>[12x]GGGS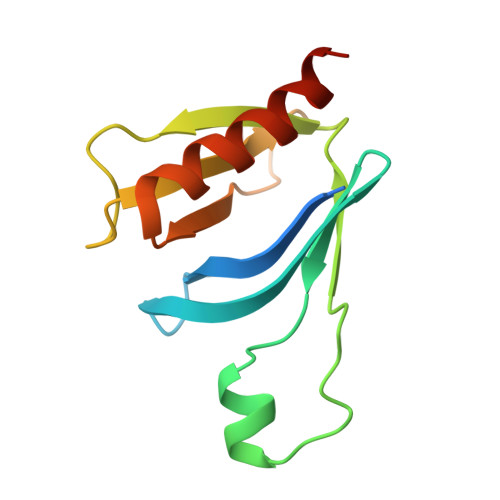GGSKKDEHKQQGELYMWDSIDQKWTRHFCAIADAKLSFSDDIEQTMEEDNPLGSLCRGILDLNTYNVVKAPQGKNQKSFVFILEPKQQGDPPVEFATDKVEELFEWFQSIREITWKIDTK Defense-associated sirtuin 2 (DSR2) systems are widely distributed across prokaryotic genomes, providing robust protection against phage infection. DSR2 recognizes phage tail tube proteins and induces abortive infection by depleting intracellular NAD+, a process that is counteracted by another phage-encoded protein, DSR Anti Defense 1 (DSAD1). Each DSR2 protomer consists of a conserved N-terminal Sirtuin (SIR2) domain, a C-terminal domain (CTD) and a middle domain (MD). DSR2 assembles into an elongated tetramer, with four NADase catalytic modules clustered in the center and the regulatory-sensing modules distributed at four distal corners.

To avoid the cytotoxicity of DSR2 NADase activation, we co-expressed a catalytic mutant DSR2H171A lacking NADase activity with Tube protein, and successfully purified the DSR2H171A-Tube complex. To gain a better understanding of how DSR2 recognizes the phage tail tube protein, we reconstituted the Tube-bound complex DSR2H171A-Tube and determined its cryo-EM structure at a resolution of 3.58 Å. The structure of the DSR2H171A-Tube complex shows the same “bone-shaped” architecture as the apo DSR2 tetramer and reveals a 4:4 assembly with a tetrameric core of DSR2 subunits braced on each corner by a Tube protein. When the hexameric Tube is superimposed on the structure of the DSR2-Tube complex, a clash between the Tube hexamer and DSR2 is observed, explaining why only the monomeric Tube protein and not the hexameric Tube is able to activate the NADase activity of DSR2. Each Tube protein binds to two DSR2 proteins on the same side (3152.65 Å2 for DSR2(a) and 886.14 Å2 for DSR2(b), respectively). In the Tube-DSR2 surface, the phage tube protein forms intermolecular interactions with both the middle domain and the C-terminal domain of DSR2. The Tube-DSR2 interactions are mainly mediated by a large hydrophobic area on the middle domain. On another binding site (Site2), the loop (aa 35-55) of Tube is completely inserted into the ring of the C-terminal circular solenoid structure DSR2, forming strong hydrophobic interactions. For each DSR2 protomer, binding of Tube proteins induces significant changes in the conformation and relative positions of the SIR2 and CTD domains, with an RMSD of 4.1 Å over 984 aligned Cα atoms. Upon interaction with the Tube protein, the circular solenoid lid of the CTD in DSR2 undergoes a downward rotation of approximately 30°, firmly attaching to the Tube.

>[4x]VKVDLESKRYGEKLKEVFLMLDNNVVECIKEITESSRNGKLVFFVGAGVSTLSDYPQWWRLVDKYHEELYGSPKKGNYSSDEYLRIPQIFYNVKGEMAFDGILKDFFQVDKPTNPIHDKILAMNPAHVITTNYDNLIDTACWKRGKYFSVISAEEDVANATSSRYLLKVAGDFRKGFKGENVVLKEDDYLNYDQNYPLISNLMKTIIATHTIVFIGYGLGDYNINMLLNWVRKLQKDSFHKPFFIRTDPSPIENETLIYYENKGLRIIDAASLIDSNEYDYLERYSAVMDLLIESQENKFITKDDEVIDYIYGKISPLFALQYIRKIDLKHVFEYDYHFEVNGTVVRHKNKGFGYMERFFELKESCDERSKLSKKQYERFNALFNFFEKNGVICMAKDAGTLNTSIEINSLAYHGKYDVMKKFIEEQSVSIEDDYKKAFFLACLGRWEESYDLYSNIILNSIDESNGCVYYLSQINRYRIYQSITQAVTQFNGLGLLTFGRHYKPFTDEFLARIEREMTNFNIDDLFNGMPFEFQKKYKILEFLSDNQFLYDDTVKLFELTNKVRSEMSEGSYSFGMSSDIVVLLRLYDNLRFLYENCLWSVSFHEFHQYIRNSMSLLIEKAEYERTRDIDELGFSFFGKKSGFFMEYYDFVNISRHFKIDDIKNLERSCSIDKIRFGEQEKIEEYLVGIAEEITKQFSANGMNVVFYTQFISEAKAALYFAKYVKLSEEGLGKIVKALLFYFPERDLDIGKRYVWLERLTKCNELPKSIISIIDDFLVLQAEKHIDQNYSEVSSNGLYSRDYGALIKHFEKNFISKRLSEITLCLTQDKQKQIDFLFKLLPLLSTNAKSHLLSFKSVENINDLMNGIRIGLIDEFTPEHEELIIEYLETRKVNYIVEKEKGIQTFSSNDYMSTFGIWYFLEEINNSKMEEFIGMDDQYDFFVDPENFDYKKFIPSWLKNYNDKLLGKIAGNKHMKHHVIEVLKERVKNSNDKRYLEILMNYFI;>MKTVIQDTADVYFKRKSDGKLVFTAEAQTASFSQAISEEKLRGGIGNKPLYILKSEKEINLTVKNAFFDLEWLAMTQGETIQEETKVKVFDREHGLIVDDTNKVTLKGKPVSDVTFYNKKGLTYKIAVSTDGTYTIPTAFAAAKDKLTAVYQIEKVGRRLAIKASKFSERYEVEYRTIAYNPDTEEVYSDIYIQFPNVSPSGEFEMSLENGNALAPEIKFEALADTDTDEMAVVIEASRDENTAAPVEDTTGSTQSSDLGGTTE[4x]> PAKKPLTKIVSHLLVAEPDKLYAMPPPGMPEGDIKALTTLCDLADRELVVIIGWAKHIPGFSSLSLGDQMSLLQSAWMEILILGIVYRSLPYDDKLVYAEDYIMDEEHSRLAGLLELYRAILQLVRRYKKLKVEKEEFVTLKALALANSDSMYIEDLEAVQKLQDLLHEALQDYELSQRHEEPWRTGKL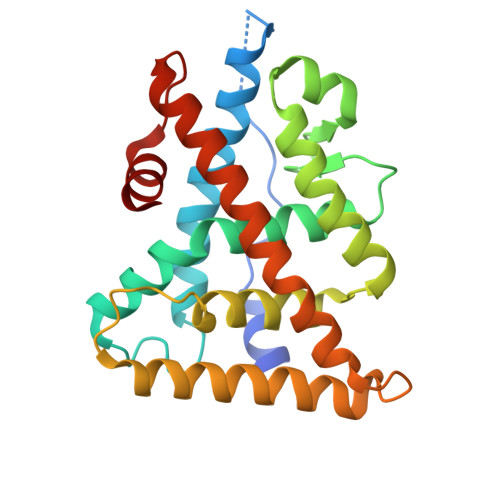LLTLPLLRQTAAKAVQHFYSVKLQGKVPMHKLFLEMLEAK> GEFDEDLEELCPVCGDKVSGYHYGLLTCESCKGFFKRTVQNNKRYTCIENQNCQIDKTQRKR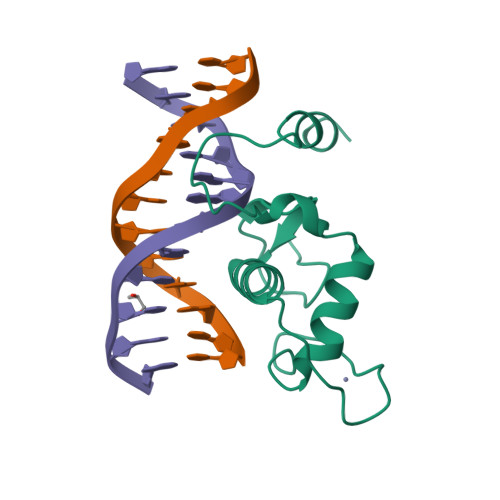CPYCRFQKCLSVGMKLEAVRADRMRGGRNKFGPMYKRDRALKQQKKALIR2-{4-[(4-imidazo[1,2-a]pyridin-3-ylpyrimidin-2-yl)amino]piperidin-1-yl}-N-methylacetamide | C19 H23 N7 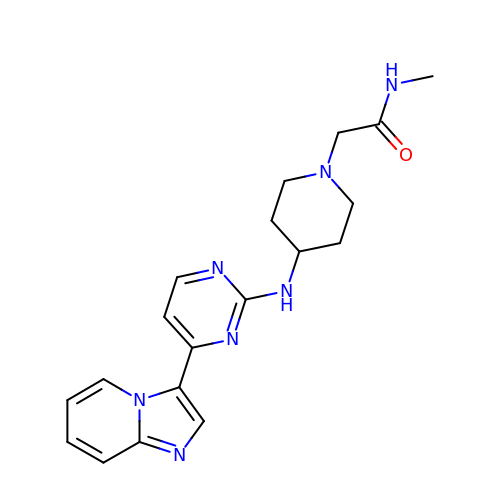O | AJLILYAPRHIFAS-UHFFFAOYSA-N>[2x]GSMMLSLNNLQNIIYNPVIPFVGTIPDQLDPGTLIVIRGHVPSDADRFQVDLQNGSSVKPRADVAFHFNPRFKRAGCIVCNTLINEKWGREEITYDTPFKREKSFEIVIMVLKDKFQVAVNGKHTLLYGHRIGPEKIDTLGIYGKVNIHSIGFSFSSHMRLPFAARLNTPMGPGRTVVVKGEVNANAKSFNVDLLAGKSKDIALHLN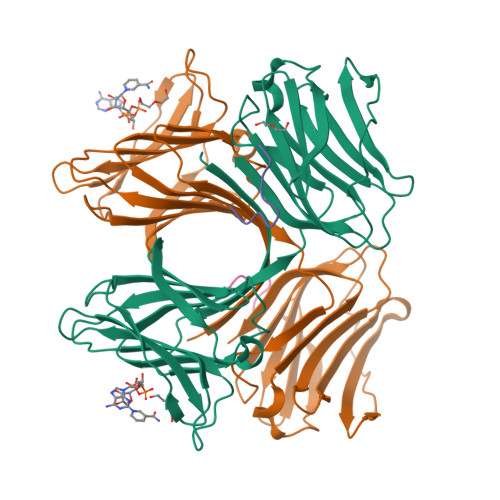PRLNIKAFVRNSFLQESWGEEERNITSFPFSPGMYFEMIIYCDVREFKVAVNGVHSLEYKHRFKELSSIDTLEINGDIHLLEVRSW;>[2x]PGLAYGNPYSGIQE3-(4-PIPERIDYL)-N-[2-(TRIFLUOROMETHOXY)PHENYL]SULFONYL-PROPANAMIDE 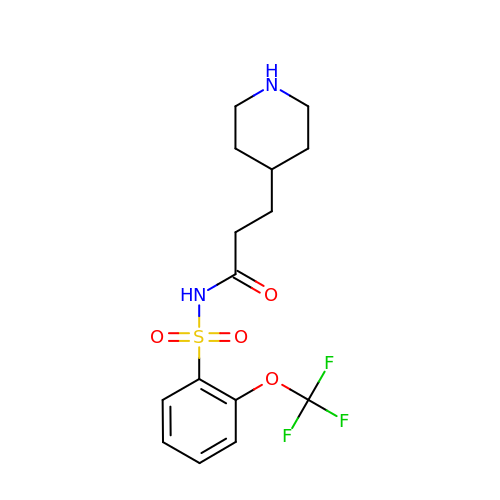| C15 H19 F3 N2 O4 S | GEYPQDLUWKGWHC-UHFFFAOYSA-N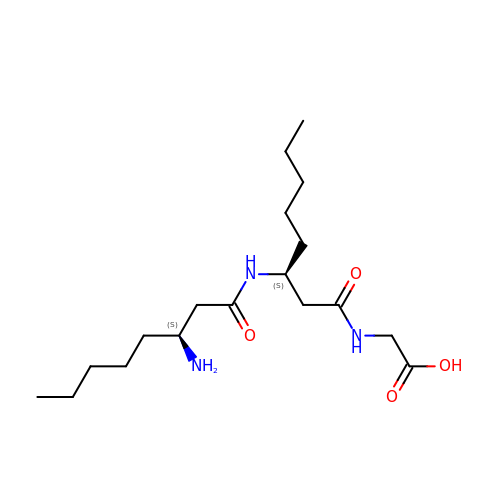N-{(3S)-3-[(3S)-3-aminooctanamido]octanoyl}glycine | C18 H35 N3 O4 | XLQURZDVPKKPRC-GJZGRUSLSA-N> ADNLAEFHVQNQECDSCHTPDGELSNDSLTYENTQCVSCHGTLAEVAETTKHEHYNAHASHF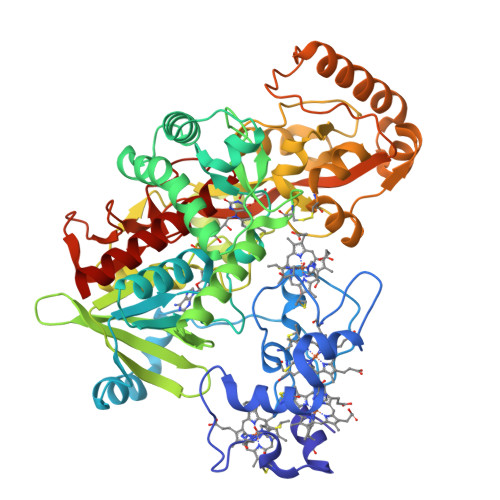PGEVACTSCHSAHEKSMVYCDSCHSFDFNMPYAKKWLRDEPTIAELAKDKSERQAALASAPHDTVDVVVVGSGGAGFSAAISATDSGAKVILIEKEPVIGGNAKLAAGGMNAAWTDQQKAKKITDSPELMFEDTMKGGQNINDPALVKVLSSHSKDSVDWMTAMGADLTDVGMMGGASVNRAHRPTGGCGVGAHVVQVLYDNAVKRNIDLRMNTRGIEVLKDDKGTVKGILVKGMYKGYYWVKADAVILATGGFAKNNERVAKLDPSLKGFISTNQPGAVGDGLDVAENAGGALKDMQYIQAHPTLSVKGGVMVTEAVRGNGAILVNREGKRFVNEITTRDKASAAILAQTGKSAYLIFDDSVRKSLCKIDKYIGLGVAPTADSLVKLGKMEGIDGKALTETVARYNSLVSSGKDTDFERPNLPRALNEGNYYAIEVTPGVHHTMGGVMIDTKAEVMNAKKQVIPGLYGAGEVTGGVHGANRLGGNAISDIITFGRLAGEEAAKYSKKN>[4x]MILLDTNVISEPLRPQPNERVVAWLDSLILEDVYLSAITVAEMRLGVALLLNGKKKNVLHERMEQSILPLFAGRILPFDEPVAA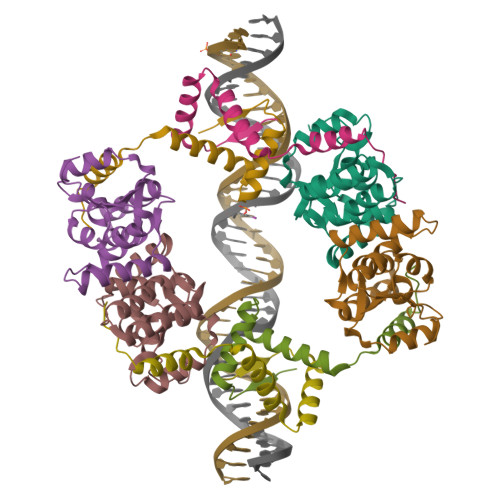IYAQIRSYAKTHGKEIAAADGYIAATAKQHSMTVATRDTGSFFAADVAVFNPWHLEHHHHHH;>[4x]ASVVIRNLSEATHNAIKFRARAAGRSTEAEIRLILDNIAKAQQTVRLGSMLASIGQEIGGVELEDVRGRNTDNEVSL> SIYNSFYVYCKGPCQRVQPGKLRVQCSTCRQATLTLTQGPSCWDDVLIPNRMSGECQSPHCPGTSAEFFFKCGAHPTSDKETSVALHLIATNSRNITCITCTDVRSPVLVFQCNSRHVICLDCFHLYCVTRLNDRQFVHDPQLGYSLPCVAGCPNSLIKELHHFRILGEEQYNRYQQYGAEECVLQMGGVLCPRPGCGAGLLPEPDQRKVTCEGGNGLGCGFAFCRECKEAYHEGECSAVFEASGTTTQAYRVDERAAEQARWEAASKETIKKTTKPCPRCHVPVEKNGGCMHMKCPQPQCRLEWCWNCGCEWNRVCMGDHWFDV

The covalent attachment of ubiquitin to specific protein substrates is achieved through the action of E3 ubiquitin ligases. Parkin has been proposed to function as a RBR ligase such that it encompasses both of the major classes of E3 ligase in one protein. Our structural, biochemical and cellular data indicate that Parkin functions as a RING/HECT hybrid. Parkin likely binds E2 through a conserved structural motif on a canonical RING domain, and also functions through a HECT-like active site cysteine whose activity can be regulated through interaction between the R0 and R2 domains.

To gain insight into the RBR class of E3 ligase, we grew crystals of Parkin-R0RBR (residues 141–465) that includes RING 0 (R0) and the RBR domains. We solved two structures of Parkin to determine if there were any notable structural differences between the sequence of Parkin originally reported (containing P223) and the updated sequence (S223). Overall the two structures were extremely similar; however, the loop containing S223 was visible in Parkin-R0RBR but not in the P223 structure. Aspects discussed in this paper were indistinguishable for Parkin with S or P at position 223; The structure discussion focuses on the S223 protein. The R0 domain (residues 141–216) is a previously unobserved domain fold (based on Dali), while R1 (residues 228–328) shows the classical cross-brace arrangement and Zn coordination of canonical RING domains. R2 contains the proposed catalytic cysteine (C431) that is near the hydrophobic interface with R0. The R0:R2 interface is unique to Parkin as it involves sequences within R0 as well as the C-terminus of R2 that are distinct from other RBR ligases. In our structure, F463 is involved in critical hydrophobic interactions predicted to contribute to integrity of R0:R2 interface. As is common for DUBs711 in our structure C431 and H433 are not well aligned for catalysis and implies that a conformational rearrangement must occur for catalysis to take place. The R1:IBR domain group contains the putative E2-binding site, which appears to be obstructed by a portion of the IBR, that we have designated the ‘tether’.>MSVEKIPGYTYGETENRAPFNLEDLKLLKEAVMFTAEDEEYIQKAGEVLEDQVEEILDTWYGFVGSHPHLLYYFTSPDGTPNEKYLAAVRKRFSRWILDTSNRSYDQAWLDYQYEIGLRHHRTKKNQTDNVESVPNIGYRYLVAWIYPITATMKPFLARKGHTPEEVEKMYQAWFKATTLQVALWSYPYVKYGDF[2x]

Pgbs are single-domain archaeal heme proteins that are related to the N-terminal domain of globin-coupled sensors (GCSs). In addition to the typical 3-on-3 helical fold found in many globins, the heme group in MaPgb* is completely buried in the protein matrix by a 20-residue N-terminal loop followed by an extra Z-helix and some inter-helical loops with a previously characterized functional role. Thus, the heme is only accessible through two orthogonal tunnels located at the B/G and B/E interfaces (named tunnel 1 and tunnel 2, respectively). Although MaPgb* assembles into a homodimer in solution, this structure does not result in cooperative CO binding.

The mutant protein solutions were equilibrated against a precipitant solution containing 10% (v/v) isopropanol, 20% (v/v) PEG 4000, 0.1 M Na-Hepes (pH 7.5), 0.02 M potassium ferricyanide, and 0.01 M KCN at 277 K. The crystals diffracted to 1.6 Å and 2.2 Å resolution for the Phe(93)E11Tyr(III)-cyanide and Phe(145)G8Trp(III)-cyanide mutants, respectively (at 100 K), using synchrotron radiation (ESRF, Grenoble, France); both crystals belong to the primitive monoclinic P21 space group. Similar considerations apply to the conserved dimeric assembly; this assembly is based on the following: a four-helix bundle built by the G- and H-helices, the H’-helix, partly the Z-helix, and the BC and FG hinges. Both ferric MaPgb* mutants have been crystallized in the presence of cyanide, which is clearly visible in the electron density of the Phe(93)E11Tyr mutant as the heme-Fe(III)-coordinated ligand but not for the Phe(145)G8Trp mutant, where the heme-Fe(III) atom appears to be free of a distal ligand. The Phe(145)G8Trp mutation results in a composite rearrangement of the heme distal site cavity, with side-chain crowding that prevents cyanide binding. In the mutant, the side-chain locations of Phe(93)E11, Trp(60)B9, and Tyr(61)B10 match those found in the native ligand-free MaPgb*(III) structure. As a result, tunnel 1 is open because the mutated Trp(145)G8 side chain is not sufficient to hinder tunnel 1. Interestingly, previous EPR experiments indicated that the cyanide derivative of the ferric MaPgb* mutant Phe(145)G8Trp can occur but always as a mixture of high-spin Fe(III) and cyanide-ligated species (EPR can only detect the ferric oxidation states of the protein). Remarkably, cyanide could not be trapped in the crystal structure. In both cases, the mutation does not alter the global structure, as indicated by the rms deviation values between 0.15 and 0.45 Å (calculated for 190 Cα atom pairs) for the structure of the cyanide derivative of ferric MaPgb* (MaPgb*(III)-cyanide) and the structure of ferrous oxygenated MaPgb* (MaPgb*(II)-O2). The kinetics of CO rebinding to Phe(145)G8Trp(II) is also very similar to that of MaPgb*(II).> SNAMRILMLGNSLTTANHMPDMLAELLTAEVRVHARGGARLAEHLNPKTRNGALTQAALANEAWDFVVMQEMSHGPATSPTAYARSVASLSEAAKAAGAQPVIYGTWPYR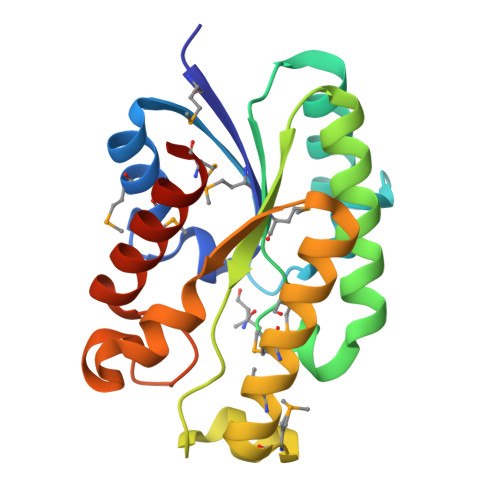AGCAKLVKLGMSHDDMSLRMAEAFAQAAADSGALLADVAAPFRAGSADELYAADGVHPSPAGSRLAALVLAETMGKGIRPW>MGFLAGKKILITGLLSNKSIAYGIAKAMHREGAELAFTYVGQFKDRVEKLCAEFNPAAVL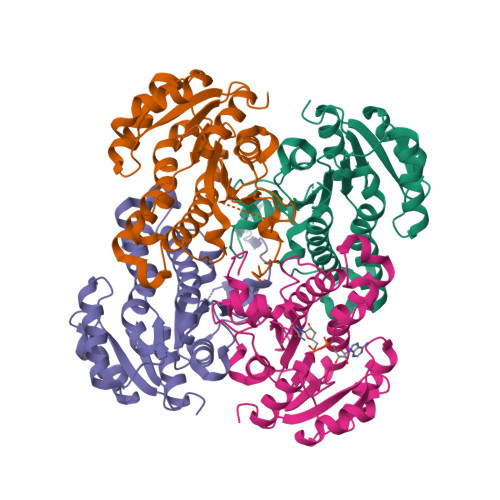PCDVISDQEIKDLFVELGKVWDGLDAIVHSIAFAPRDQLEGNFIDCVTREGFSIAHDISAYSFAALAKEGRSMMKNRNASMVALTYIGAEKAMPSYNTMGVAKASLEATVRYTALALGEDGIKVNAVSAGPIKTLAASGISNFKKMLDYNAMVSPLKKNVDIMEVGNTVAFLCSDMATGITGEVVHVDAGYHCVSMGNVLLEHHHHHH[4x]>AMADIGSMGDPLTWSKALKKLEKVTVQGSQKLTTGNCNWALSLVDLFHDTNFVKEKDWQLRDVIPLLEDVTQTLSGQEREAFERTWWAISAVKMGLQINNVVDGKASFQL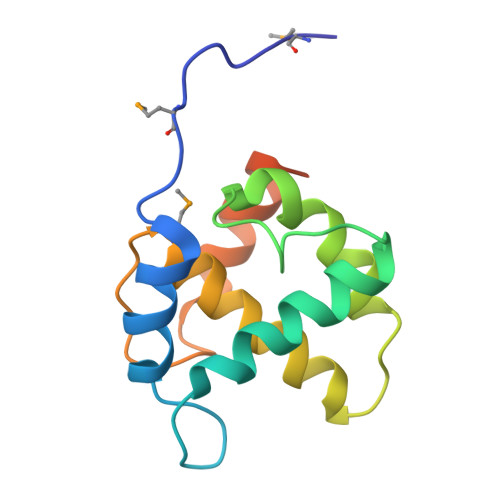LRAKYEKKTANKKQSEPSEEY[2x]2-[4-(4-cyanophenyl)-3-[(4-pyridin-2-ylpiperazin-1-yl)methyl]phenoxy]acetic 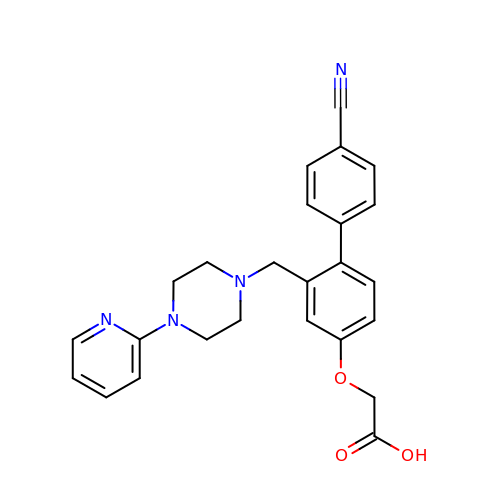acid | C25 H24 N4 O3 | AKNGILSRJWORBU-UHFFFAOYSA-N> DVSFRLSGADPSSYGMFIKDLRNALPHTEKVYNIPLLLPSVSGAGRYLLMHLFNYDGNTITVAVDVTNVYIMGYLALTTSYFFNEPAADLASQYVFRSARRKITLPYSGNYERLQIAAGKPREKIPIGLPALDTAISTLLHYDSTA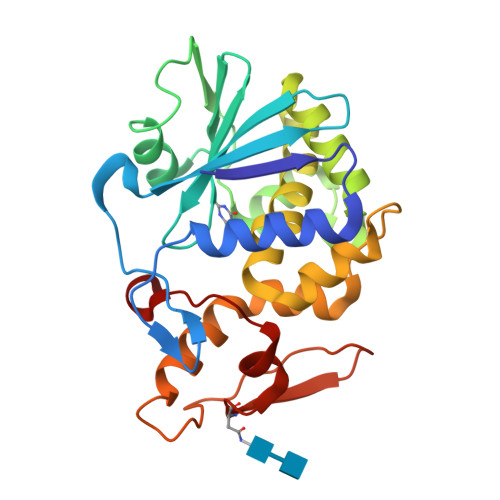AAGALLVLIQTTAEAARFKYIEQQIQERAYRDEVPSSATISLENSWSGLSKQIQLAQGNNGVFRTPTVLVDSKGNKVQITNVTSNVVTSNIQLLLNTKNI>[2x]GPL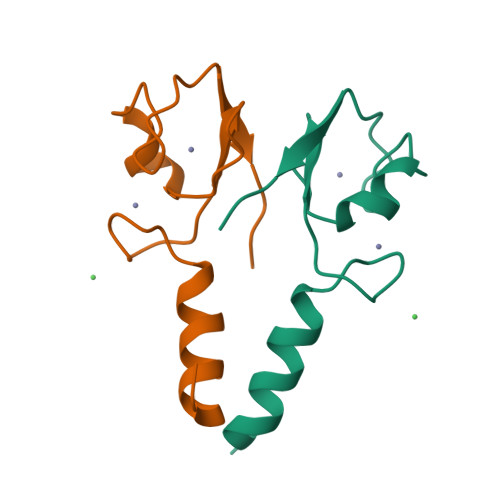GSTSLQKEISTEEQLRRLQEEKLCKICMDRNIAIVFVPCGHLVTCKQCAEAVDKCPMCYTVITFKQKILMS>MNLKDKILGVAKELFIKNGYNATTTGEIVKLSESSKGNLYYHFKTKENLFLEILNIEESKWQEQWKKEQIKAKTNREKFYLYNELSLTTEYYYPLQNAIIEFYTEYYKTNSINEKMNKLENKYIDAYHVIFKEGNLNGEWSINDVNAVSKIAANAVNGIVTFTHEQNINERIKLMNKFSQIFLNGLSKHHHHHH[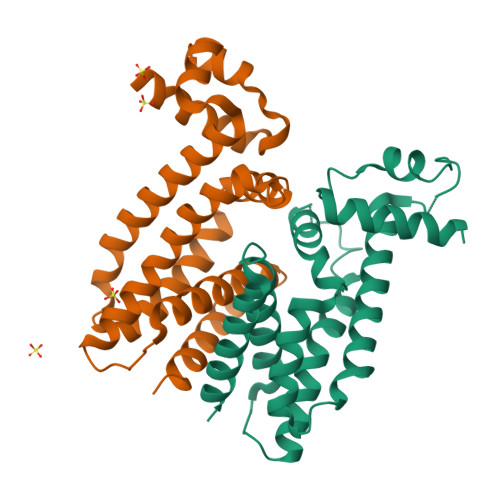4x]> MKHHHHHHSAGLEVLFQGPGTGSEFMMFGKKKNNGGSSTARYSAGNKYNTLSNNYALSAQQLLNASKIDDIDSMMGFERYVPPQYNGRFDAKDIDQIPGRVGWLTNMHATLVSQETLSSGSNGGGNSNDGERVTTNQGISGVDFYFLDEEGGSFKSTVVYDPYFFIACNDESRVNDVEELVKKYLESCLKSLQIIRKEDLTMDNHLLGLQKTLIKLSFVNSNQLFEARKLLRPILQDNANNNVQRNIYNVAANGSEKVDAKHLIEDIREYDVPYHVRVSIDKDIRVGKWYKVTQQGFIEDTRKIAFADPVVMAFAIATT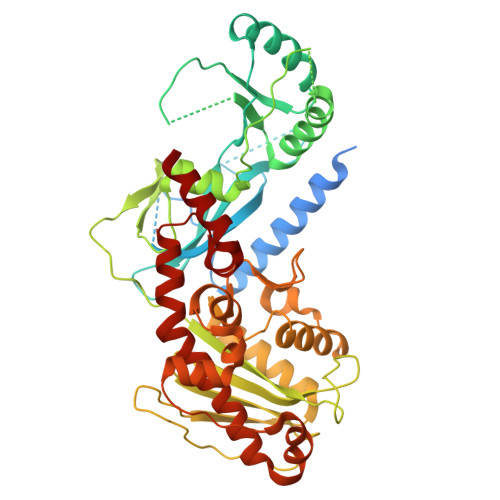KPPLKFPDSAVDQIMMISYMIDGEGFLITNREIISEDIEDFEYTPKPEYPGFFTIFNENDEVALLQRFFEHIRDVRPTVISTFNGDFFDWPFIHNRSKIHGLDMFDEIGFAPDAEGEYKSSYCSHMDCFRWVKRDSYLPQGSQGLKAVTQSKLGYNPIELDPELMTPYAFEKPQHLSEYSVSDAVATYYLYMKYVHPFIFSLCTIIPLNPDETLRKGTGTLCEMLLMVQA> PSSVY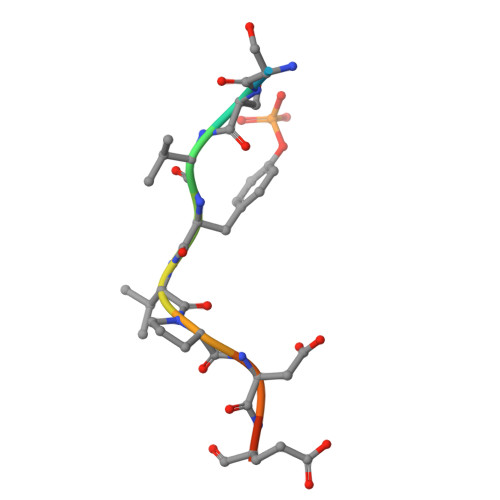VPDEWE> GSAMGSASTSGNPFQANVEMKTFMERFNLTHHHQSGIYVDLGQDKEVDGTLYREPAGLCPIWGKHIELQQPDRPPYRNNFLEDVPTEKEYKQSGNPLPGGFNLNFVTPSGQRISPFPMELLEKNSNIKASTDLGRCAEFAFKTVAMDKNNKATKYRYPFVYDSKKRLCHILAVSMQLMEGKKYCSVKGEPPDLTWYCFKPRKSVTENHHLIYGSAYVGENPDAFISKCPNQALRGYRFGVWKKGRCLDYTELTD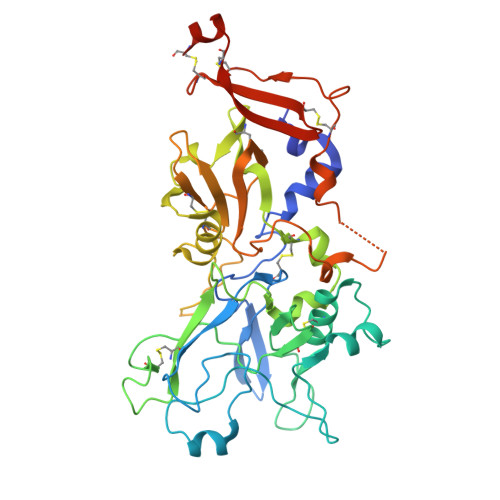TVIERVESKAQCWVKTFENDGVASDQPHTYPLTSQASWNDWWPLHQSDQPHSGGVGRNYGFYYVDTTGEGKCALSDQVPDCLVSDSAAVSYTAAGSLSEETPNFIIPSNPSVTPPTPETALQCTADKFPDSFGACDVQACKRQKTSCVGGQIQSTSVDCTADEQNECGSNTAAALVPR6-chloranyl-10-methyl-1,2,3,4-tetrahydroacridin-10-ium-9-amine | C14 H16 Cl N2 | 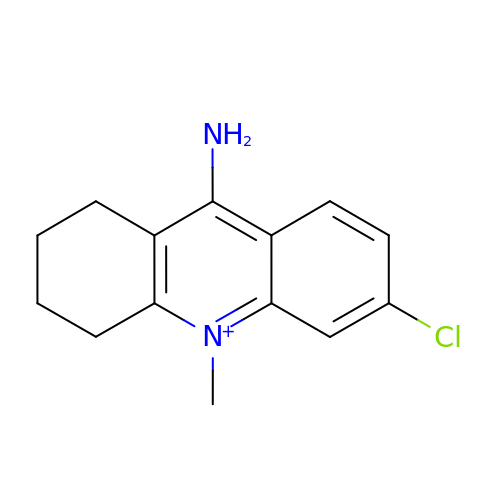NNLSQYGKFPZYHI-UHFFFAOYSA-O> SMAAFKPNPINYILGLAIGIASVGWAMVEIDEEENPIRLIDLGVRVFERAEVPKTGDSLAMARRLARSVRRLTRRRAHRLLRARRLLKREGVLQAADFDENGLIKSLPNTPWQLRAAALDRKLTPLEWSAVLLHLIKHRGYLSQRKNEGETADKELGALLKGVANNAHALQTGDFRTPAELALNKFEKESGHIRNQRGDYSHTFSRKDLQAELILLFEKQKEFGNPHVSGGLKEGIETLLMTQRPALSGDAVQKMLGHCTFEPAEPKAAKNTYTAERFIWLTKLNNLRILEQ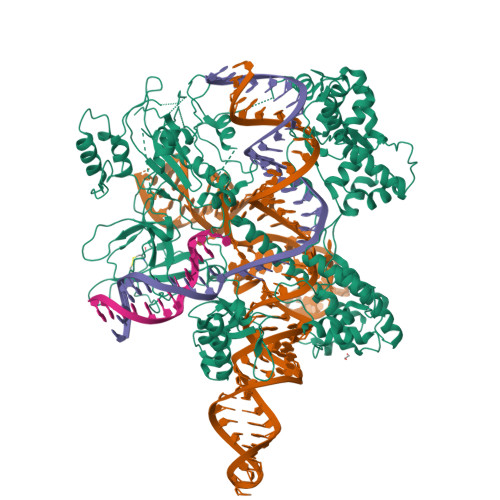GSERPLTDTERATLMDEPYRKSKLTYAQARKLLGLEDTAFFKGLRYGKDNAEASTLMEMKAYHAISRALEKEGLKDKKSPLNLSSELQDEIGTAFSLFKTDEDITGRLKDRVQPEILEALLKHISFDKFVQISLKALRRIVPLMEQGKRYDEACAEIYGDHYGKKNTEEKIYLPPIPADEIRNPVVLRALSQARKVINGVVRRYGSPARIHIETAREVGKSFKDRKEIEKRQEENRKDREKAAAKFREYFPNFVGEPKSKDILKLRLYEQQHGKCLYSGKEINLVRLNEKGYVEIDAALPFSRTWDDSFNNKVLVLGSENQNKGNQTPYEYFNGKDNSREWQEFKARVETSRFPRSKKQRILLQKFDEDGFKECNLNDTRYVNRFLCQFVADHILLTGKGKRRVFASNGQITNLLRGFWGLRKVRAENDRHHALDAVVVACSTVAMQQKITRFVRYKEMNAFDGKTIDKETGKVLHQKTHFPQPWEFFAQEVMIRVFGKPDGKPEFEEADTPEKLRTLLAEKLSSRPEAVHEYVTPLFVSRAPNRKMSGAHKDTLRSAKRFVKHNEKISVKRVWLTEIKLADLENMVNYKNGREIELYEALKARLEAYGGNAKQAFDPKDNPFYKKGGQLVKAVRVEKTQESGVLLNKKNAYTIADNGDMVRVDVFCKVDKKGKNQYFIVPIYAWQVAENILPDIDCKGYRIDDSYTFCFSLHKYDLIAFQKDEKSKVEFAYYINCDSSNGRFYLAWHDKGSKEQQFRISTQNLVLIQKYQVNELGKEIRPCRLKKRPPVR The nuclear envelope partitions nuclear components from the cytoskeleton, thereby necessitating their mechanical coupling across the nuclear envelope to enable cytoskeletal function in the structure and positioning of nuclear contents. This is achieved by the Linker of Nucleoskeleton and Cytoskeleton (LINC) complex, which traverses the nuclear envelope and binds to cytoskeletal and nuclear structures to mediate force transduction between these partitioned components (Haque et al., 2006; Crisp et al., 2006; Lee and Burke, 2018; Meinke and Schirmer, 2015). The LINC complex is formed of SUN (Sad1 and UNC84 homology) domain and KASH (Klarsicht, ANC-1, and Syne homology) domain proteins, which interact immediately below the outer nuclear membrane, through complex formation between their C-terminal eponymous SUN and KASH domains. Thus, the LINC complex axis is established by a peri-nuclear SUN-KASH core interaction and mechanically couples the cytoskeleton and nuclear contents. We find that SUN-KASH complexes between SUN proteins and Nesprin-4, KASH5 and Nesprin-1 are 6:6 structures formed of constitutive interactions between two 3:3 complexes.

The SUN1-KASH4 structure was solved at a resolution of 2.75 Å and revealed a 6:6 assembly in which two globular 3:3 complexes are held in a head-to-head configuration through zinc-coordination by opposing KASH4 molecules across the 6:6 interface. SUN1-KASH4 adopts an unusual conformation in which the 6:6 complex is held together by three interface spanning zinc-sites, each coordinated by opposing KASH4 molecules. The presence of metal ions in the crystal structure was confirmed by corresponding peaks in anomalous difference electron density maps, and their identity as zinc ions that were co-purified from bacterial expression was confirmed by the spectrophotometric determination of three zinc ions per 6:6 complex in solution that were lost upon pre-incubation with EDTA. The zinc-sites are coordinated by asymmetric ligands from 381-CCSH-384 motifs of opposing KASH4 molecules, comprising C381 and C382 from one molecule, and C382 and H384 from the other, and mutation of both cysteine residues to serine was sufficient to preclude zinc-binding. The three zinc-sites form a tripod of interactions that provide the sole interface-spanning contacts between opposing 3:3 complexes. KASH1 undergoes a turn of >90° to radiate from the trimer axis, similar to the previously reported SUN2-KASH1/2 structures, whereas KASH4 and KASH5 follow the arc of the SUN1 trimer, enabling them to contribute directly to the 6:6 interface. We confirmed this hypothesis for SUN1-KASH4 through the finding that the 6:6 complex is retained upon zinc removal by pre-incubation with EDTA, likely through reversal to a KASH1-like interface in which the head-to-head interaction is mediated solely by SUN1 amino acids.

>GSGGSGGITEAQARAIVNSALKLYSQDKTGMVDFALESGGGSILSTRCSETYETKTALMSLFGIPLWYFSQSPRVVIQPDIYPGNCWAFKGSQGYLVVRLSMMIHPAAFTLEHIPKTLSPTGNISSAPKDFAVYGLENEYQEEGQLLGQFTYDQDGESLQMFQALKRPDDTAFQIVELRIFSNWGHPEYTCLYRFRVHGEPVK[6x];>[6x]GSMASGGPCCSHARIPRTPYLVLSYVNGLPPV>[6x]MAQQSTKNETALLVAKSAKSALQDFNHDYSKSWTFGDKWDNSNTMFETFVNKYLFPKINETLLIDIALGNRFNWLAKEQDFIGQYSEEYVIMDTVPINMDLSKNEELMLKRNYPRMATKLYGNGIVKKQKFTLNNNDTRFNFQTLADATNYALGVYKKKISDINVLEEKEMRAMLVDYSLNQLSETNVRKATSKEDLASKVFEAILNLQNNSAKYNEVHRA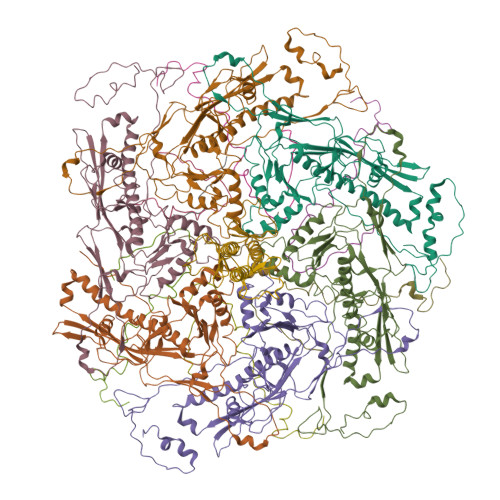SGGAIGQYTTVSKLKDIVILTTDSLKSYLLDTKIANTFQIAGIDFTDHVISFDDLGGVFKVTKEFKLQNQDSIDFLRAYGDYQSQLGDTIPVGAVFTYDVSKLKEFTGNVEEIKPKSDLYAFILDINSIKYKRYTKGMLKPPFHNPEFDEVTHWIHYYSFKAISPFFNKILITDQDVNPKPEEELQE;>[6x]MYEGNNMRSMMGTSYEDSRLNKRTELNENMSIDTNKSEDSYGVQIHSLSKQSFTGDVEEE2-KETOBUTYRIC ACID | C4 H6 O3 | 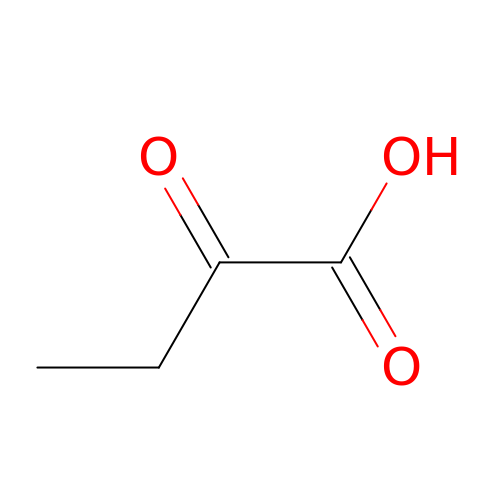TYEYBOSBBBHJIV-UHFFFAOYSA-N>TLPKRVKIVEVGPMDGLQNEKNIVSTPVKIKLIDMLSEAGLSVIETTSFVSPKWVPQMGDHTEVLKGIQKFPGINYPVLTPNLKGFEAAVAAGAKEVVIFGAASELFTKKNINCSIEESFQRFDAILK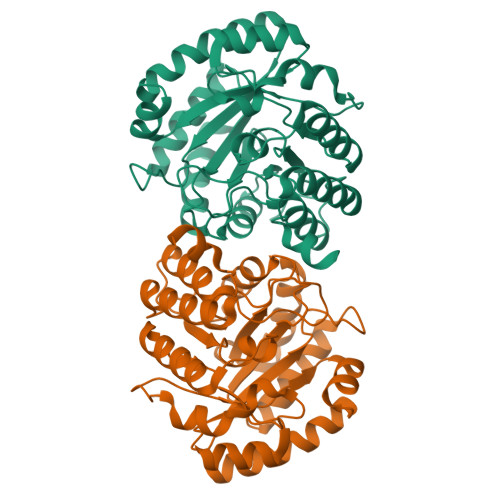AAQSANISVRGYVSCALGCPYEGKISPAKVAEVTKKFYSMGCYEISLGDTIGVGTPGIMKDMLSAVMQEVPLAALAVHCHDTYGQALANTLMALQMGVSVVDSSVAGLGGCPYAQGASGNLATEDLVYMLEGLGIHTGVNLQKLLEAGNFICQALNRKTSSKVAQATCKL[6x]> G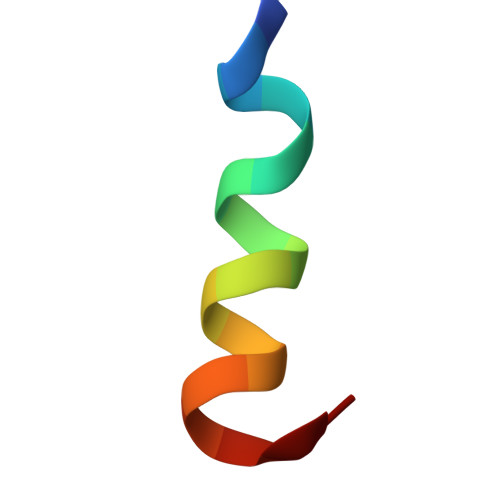PLSDNEEFENVVKNGH> MANVSKKVSWSGRDRDDEEAAPLLRRTARPGGGTPLLNGAGPGAARQSPRSALFRVGHMSSVELDDELLDPDMDPPHPFPKEIPHNEKLLSL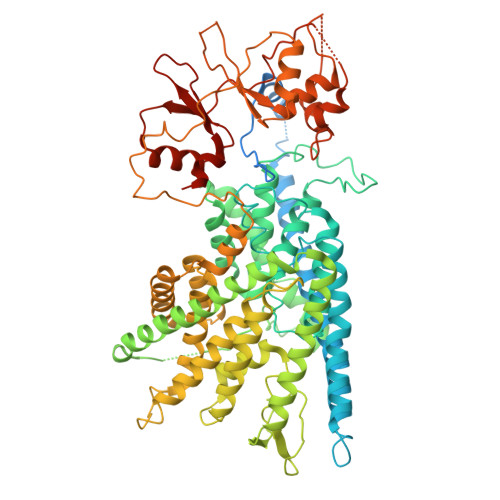KYESLDYDNSENQLFLEEERRINHTAFRTVEIKRWVICALIGILTGLVACFIDIVVENLAGLKYRVIKGNIDKFTEKGGLSFSLLLWATLNAAFVLVGSVIVAFIEPVAAGSGIPQIKCFLNGVKIPHVVRLKTLVIKVSGVILSVVGGLAVGKEGPMIHSGSVIAAGISQGRSTSLKRDFKIFEYFRRDTEKRDFVSAGAAAGVSAAFGAPVGGVLFSLEEGASFWNQFLTWRIFFASMISTFTLNFVLSIYHGNMWDLSSPGLINFGRFDSEKMAYTIHEIPVFIAMGVVGGVLGAVFNALNYWLTMFRIRYIHRPCLQVIEAVLVAAVTATVAFVLIYSSRDCQPLQGGSMSYPLQLFCADGEYNSMAAAFFNTPEKSVVSLFHDPPGSYNPLTLGLFTLVYFFLACWTYGLTVSAGVFIPSLLIGAAWGRLFGISLSYLTGAAIWADPGKYALMGAAAQLGGIVRMTLSLTVIMMEATSNVTYGFPIMLVLMTAKIVGDVFIEGLYDMHIQLQSVPFLHWEAPVTSHSLTAREVMSTPVTCLRRREKVGVIVDVLSDTASNHNGFPVVEHADDTQPARLQGLILRSQLIVLLKHKVFVERSNLGLVQRRLRLKDFRDAYPRFPPIQSIHVSQDERECTMDLSEFMNPSPYTVPQEASLPRVFKLFRALGLRHLVVVDNRNQVVGLVTRKDLARYRLGKRGLEELSLAQT2-DECENOYL N-ACETYL 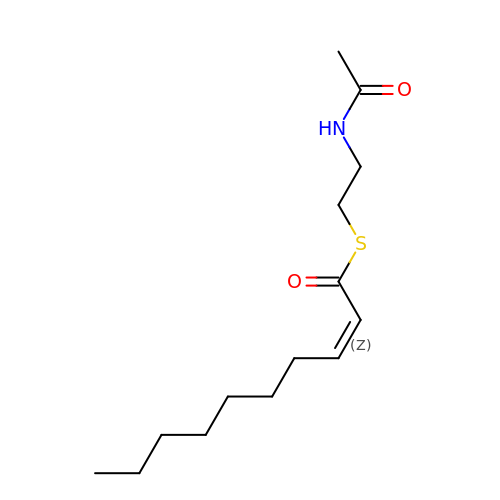CYSTEAMINE | C14 H25 N O2 S | HYDKTIAWESXLEF-KTKRTIGZSA-N>XELLKKLL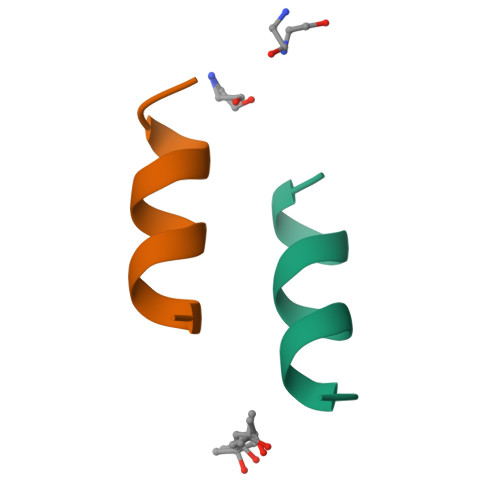EELKG[2x]> GPDAEKTLNHLISGFETFEKKINYRFKNKAYLLQAFTHASYHYNTITDCYQRLEFLGDAILDYLITKHLYEDPRQHSPGVLTDLRSALVNNTIFASLAVKYDYHKYFKAVSPELFHVIDDFVKFQLEKNEMQGMDSELRRSEEDEEKEEDIEVPKAMGDIFESLAGA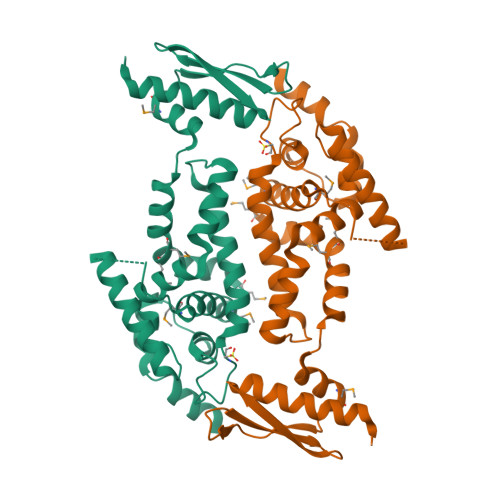IYMDSGMSLEVVWQVYYPMMQPLIEKFSANVPRSPVRELLEMEPETAKFSPAERTYDGKVRVTVEVVGKGKFKGVGRSYRIAKSAAARRALRSLKANQ>MARKYFVAANWKCNGTLESIKSLTNSFNNLDFDPSKLDVVVFPVSVHYDHTRKLLQSKFSTGIQNVSKFGNGSYTGEVSAEIAKDLNIEYVIIGHHERRKYFHETDEDVREKLQASLKNNLKAVVCFGESLEQREQNKTIEVITKQVKAFVDLIDNFDNVILVYEPLWAIGTGKTATPEQAQLVHKEIRKIVKDTCGEKQANQ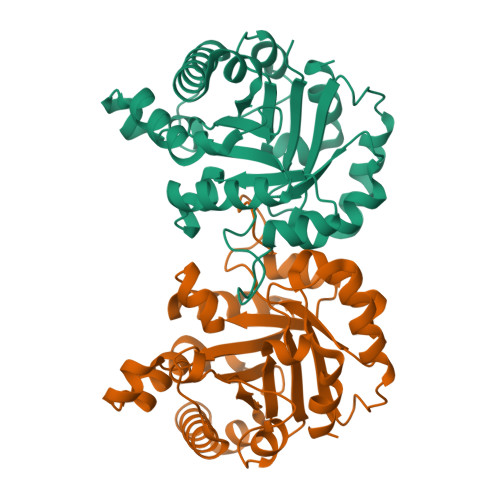IRILYGGSVNTENCSSLIQQEDIDGFLVGNASLKESFVDIIKSAM[2x]Topoisomerase V is a unique topoisomerase that combines DNA repair and topoisomerase activities. Topoisomerase V is formed by a small, ~30-kDa topoisomerase domain followed by 24 tandem helix–hairpin–helix (HhH) repeats arranged as 12 (HhH)2 domains. HhH repeats are associated with DNA lyase repair activity and 3 of the 12 (HhH)2 domains have apurinic/apyrimidinic (AP) lyase and deoxyribose-5-phosphate (dRP) lyase activities. In addition, a 97-kDa fragment of topoisomerase V mutated to have only a single AP lyase site (hereafter Topo-97(ΔRS2), see Materials and methods) was used in all crystallization trials.

The 38-bp DNA oligonucleotide was redesigned by making it symmetric from the center, with two abasic sites, and still containing overhangs (total length per strand 40 nucleotides) and led to a different crystal form. The structure of the symmetric oligonucleotide complex shows that each DNA fragment binds two protein molecules with the topoisomerase active site accessible and occupied by DNA. The two monomers are related by a twofold axis, but this axis does not coincide with the DNA sequence twofold axis creating an asymmetry in the DNA structure. The structure with a 38 bp oligonucleotide revealed that the noncrystallographic twofold axis passes through a base pair of the DNA molecule, making the 38 and 40 bp molecules sit asymmetrically in the complex; one half comprises 18 or 19 bp and the other half 19 or 20 bp for the 38 and 40 bp DNA molecules, respectively. This asymmetry translates in an asymmetry in the path of the DNA, even though the protein monomers are identical. For the 39 bp DNA, the dimer is almost perfectly symmetric with the two halves of the DNA identical. This is not the case in the 38 and 40 bp symmetric DNA complexes, where the DNA is different around the abasic site in each half. Despite the small differences in the DNA, the protein is identical in all complexes.

>[2x]MALVYDAEFVGSEREFEEERETFLKGVKAYDGVLATRYLMERSSSAKNDEELLELHQNFILLTGSYACSIDPTEDRYQNVIVRGVNFDERVQRLSTGGSPARYAIVYRRGWRAIAKALDIDEEDVPAIEVRAVKRNPLQPALYRILVRYGRVDLMPVTVDEVPPEMAGEFERLIERYDVPIDEKEERILEILRENPWTPHDEIARRLGLSVSEVEGEKDPESSGIYSLWSRVVVNIEYDERTAKRHVKRRDRLLEELYEHLEELSERYLRHPLTRRWIVEHKRDIMRRYLEQRIVECALKLQDRYGIREDVALCLARAFDGSISMIATTPYRTLKDVCPDLTLEEAKSVNRTLATLIDEHGLSPDAADELIEHFESIAGILATDLEEIERMYEEGRLSEEAYRAAVEIQLAELTKKEGVGRKTAERLLRAFGNPERVKQLAREFEIEKLASVEGVGERVLRSLVPGYASLISIRGIDRERAERLLKKYGGYSKVREAGVEELREDGLTDAQIRELKGLKTLESIVGDLEKADELKRKYGSASAVRRLPVEELRELGFSDDEIAEIKGIPKKLREAFDLETAAELYERYGSLKEIGRRLSYDDLLELGATPKAAAEIKGPEFKFLLNIEGVGPKLAERILEAVDYDLERLASLNPEELAEKVEGLGEELAERVVYAARERVESRRKSGRQERSEEEWKEWLERKVGEGRARRLIEYFGSAGEVGKLVENAEVSKLLEVPGIGDEAVARLVPGYKTLRDAGLTPAEAERVLKRYGSVSKVQEGATPDELRELGLGDAKIARILGLRSLVNARLDVDTAYELARRYGSVSAVRAAPVAELRELGLSDRAIARIAGIP4-(2-AMINOPHENYLTHIO)-BUTYLPHOSPHONIC 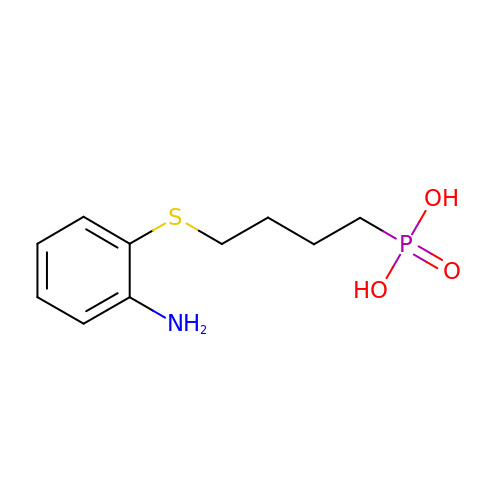ACID | C10 H16 N O3 P S | POZPBCXLYRZUTO-UHFFFAOYSA-N>[12x]SMG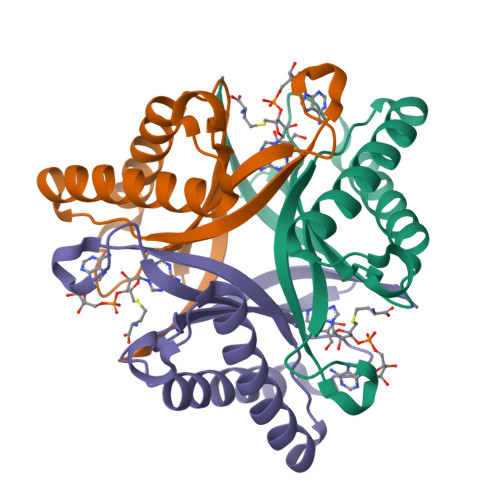KTLRFEIVSGVNKGYFHTNSQSESLDLVGGIWQKIAKEEFEKSNIYVSAVIKPSKTVYNQEWGCPENGEETVVLTGVANEEFVDDIEKWKDTVIKLAKELKNQMKQSTLTCEFIETELHYFK>ETGCPANCLCSKTDINCKKPDDGNLFPLLEGQDSRNITSIHIENWKNLQTLNAVDMELYTGLQRLTIRNSGLRNIQPRAFAKNPHLRYIDLSGNRLTTLSWQLFQTLRLFDLRLERNPFQCSCDIRWIQLWQEKGEANLQSQQLHCMNLDTAVILLRNMNITQCDLPEISVSHVNLTVREGENAVITCQGSGSPLPDVDWTVADLHSINTHQTNLQWTNVHAIQLTLVNVTSEDNGFLLTCIAENVVGMSQASVLLTVYGTKHHHHHH[2x];>ETGESPPVFIKKPVDQIGVSGGVASFVCQATGDPKPRVTWNKKGKKVNSQRFETIEFDESAGAVLRIQPLRTPRDENIYECVAQNPHGEVTVHAKLTVLREDQLPPGFPNIDMGPQLKVVERTRTATMLCAASGNPDPEITWFKDFLPVDPSTSNGRIKQLRSGGLQIESSEETDQGKYECVASNSAGVRYSSPANLYVRVRRVAPRFSILPVSHEIMPGGNVNITCVAVGSPMPYVKWMQGAEDLTPEDDMPVGRNVLELTDVKDSANYTCVAMSSLGV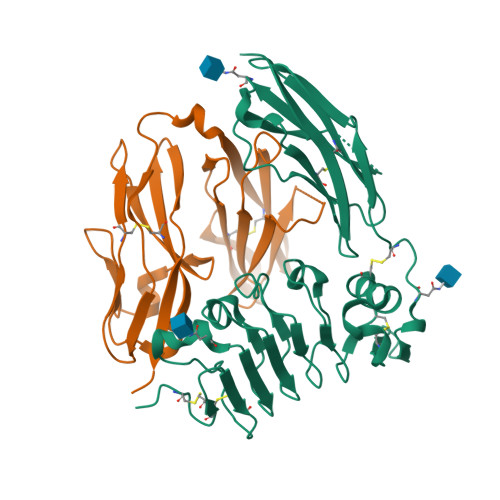IEAVAQITVKSKGHHHHHH[3x]> SGEIRPTIGQQMETGDQRFGDLVFRQLAPNVWQHTSYLDMPGFGAVASNGLIVRDGGRVLVVDTAWTDDQTAQILNWIKQEINLPVALAVVTHAHQDKMGGMDALHAAGIATYANALSNQLAPQEGMVAAQHSLTFAANG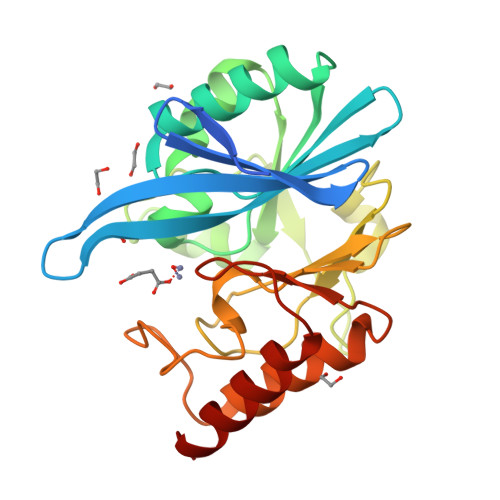WVEPATAPNFGPLKVFYPGPGHTSDNITVGIDGTDIAFGGCLIKDSKAKSLGNLGDADTEHYAASARAFGAAFPKASMIVMSHSAPDSRAAITHTARMADKLR> MSSSGTRVLIVGGSLVGLSTAVFLAHHDVPVTLVERHPGTSIHPRAVGYYPRTAELLATVGVEAPAKAAASGFEKHRTRAGVESLAGEVLFSKEELEGGDELADLTPSSLLLLPQDRLEPILRARAEELGAELRFGAELRSFTQDADGVSAVVRDADGGESVVRADYLVAADGPRSTVREALGIGREGRGVLSR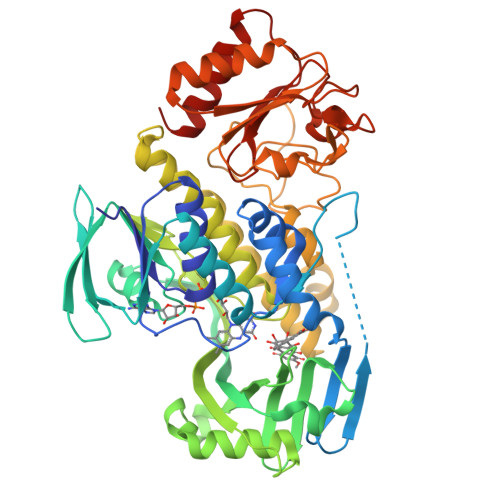HVSIAFGADFAAVLGERRYSVVHVQNDRVTGILVHDDTLTEGTLIVGYDPEKGEGLDDFTDARCAELVSAAIGSDDVAVTIRSRFPWDMAELVADAFVSDRVLVAGDAAHQIPPTGGYGANTGIADAFNLSWKLAHVLAGTAGRALLDTYDEERRPVGLYTARQGSLQLAVRSRTATEEQREAAHDAMRVTMGQAYPSGAFVADAGADPLPLTSDPRTLRGEPGTRAPYVVLERDGAPLSTLDLFGDGFVLLVGADGGSWAEAAGEAAAGLGVGIAFHRVAPDAGEGRPVDVHGRWAEAYGVGAAGAVLVRPDGIVAWRSRDGMPGGAGGRALTAALRTVLAR N-cyclopropyl-4-{8-[(thiophen-2-ylmethyl)amino]imidazo[1,2-a]pyrazin-3-yl}benzamide | C21 H19 N5 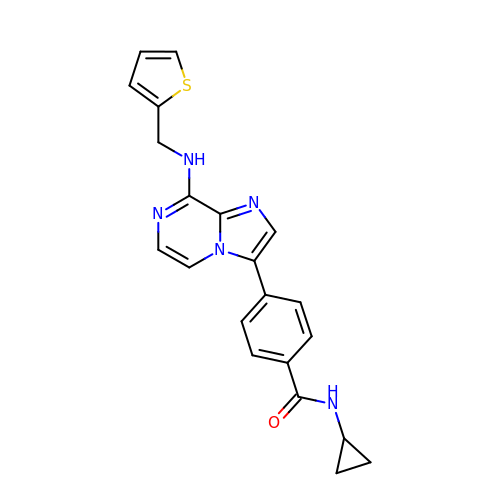O S | YUHKXKGPLTYXSO-UHFFFAOYSA-N>[2x]QLTTESMPFNVAEGKEVLLLVHNLP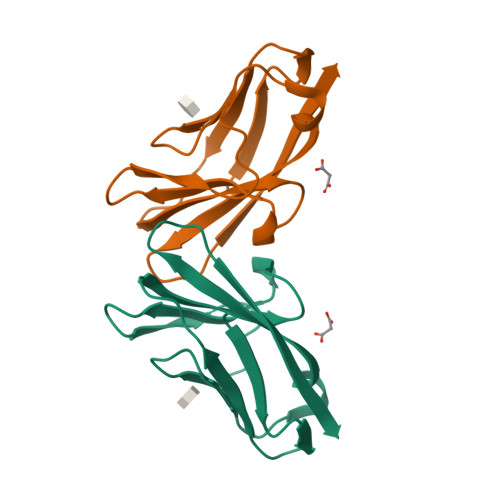QQLFGYSWYKGERVDGNRQIVGYAIGTQQATPGPANSGRETIYPNASLLIQNVTQNDTGFYTLQVIKSDLVNEAATGQFHVY3-methyl-4-phenyl-2,7-dihydropyrazolo[3,4-b]pyridin-6-one | C13 H11 N3 O | 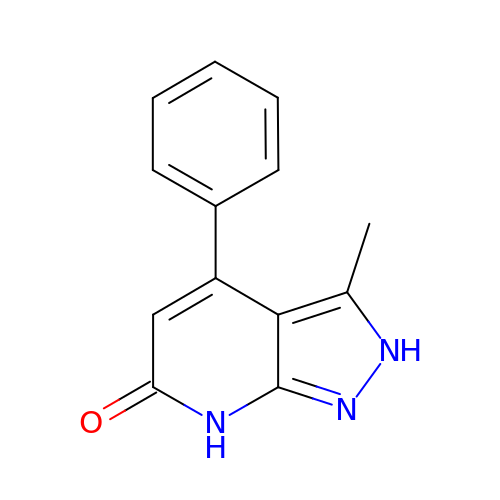LDYQYDPPCHEKQY-UHFFFAOYSA-N> MDVASSDTVYTFPDEFKLGAATASYQIEGAWDENGKGPNIWDTLTHEHPDYVVDGATGDIADDSYHLYKEDVKILKELGAQVYRFSISWARVLPEGHDNIVNQDGIDYYNNLINELLANGIEPMVTMYHWDLPQALQDLGGWPNLVLAKYSENYARVLFKNFGDRVKLWLTFNEPLTFMDGYASEIGMAPSINTPGIGDYLAAHTVIHAHARIYHLYDQEFRAEQGGKVGISLNINWCEPATNSAEDRASCENYQQFNLGLYAHPIFTEEGDYPAVLKDRVSRNSADEGYTDSRLPQFTAEEVEYIRGTHDFLGINFYTALLGKSGVEGYEPSRYRD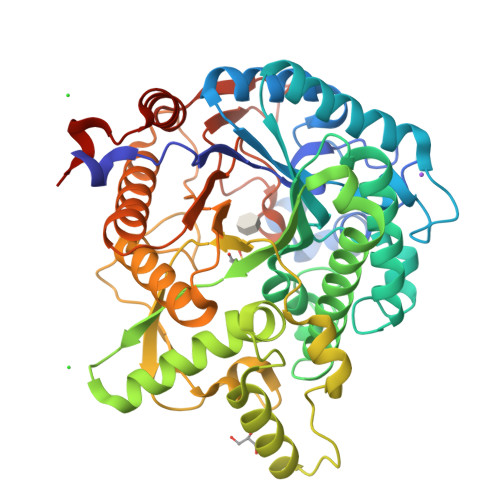SGVILTQDAAWPISASSWLKVVPWGFRKELNWIKNEYNNPPVFITENGFSDYGGLNDTGRVHYYTEHLKEMLKAIHEDGVNVIGYTAWSLMDNFEWLRGYSEKFGIYAVDFEDPARPRIPKESAKVLAEIMNTRKIPERFRDLEHHHHHH>VPNEPINWGFKRSVNHQPPDAGKQLNSLIEKYDAFYLGNTKEKTIYLTFDNGYENGYTPKVLDVLKKHRVTGTFFVTGHFVKDQPQLIKRMSDEGHIIGNHSFHHPDLTTKTADQIQDELDSVNEEVYKITGKQDNLYLRPPRGVFSEYVLKETKRLGYQTVFWSVAFVDWKINNQKGKKYAYDHMIKQAHP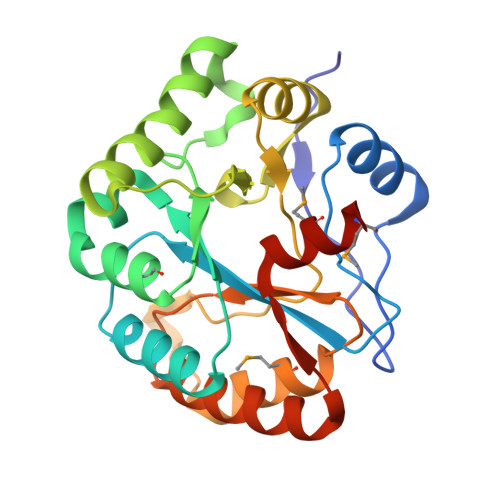GAIYLLHTVSRDNAEALDDAITDLKKQGYTFKSIDDLMFEKEMRLPSL[2x]>[4x]GSHMVKVCLFVADGTDEIEFSAPWGIFKRAEIPIDSVYVGENKDRLVKMSR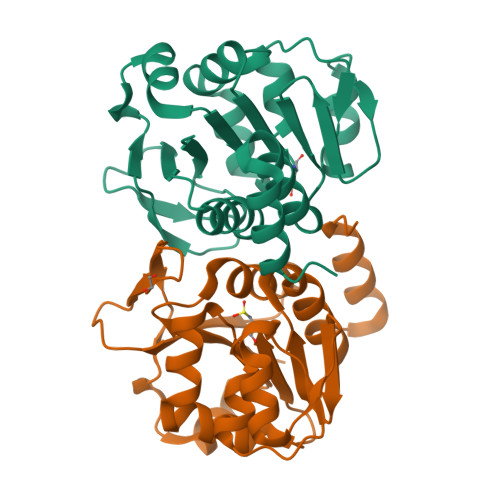DVEMYANRSYKEIPSADDFAKQYDIAIIPGGGLGAKTLSTTPFVQQVVKEFYKKPNKWIGMICAGPLTAKTSGLPNKQITGHPSVRGQLEEGGYKYLDQPVVLEENLITSQGPGTAMLFGLKLLEQVASKDKYNAVYKSLSMP>MGHHHHHHMPFAARLNTPMGPGRTVVVKGEVNANAKSFNVDLLAGKSKDIALHLNPRLNIKAFVRNSFLQESWGEEERNITSFPFSPGMYFEMIIYCDVREFKVAVNGVHSL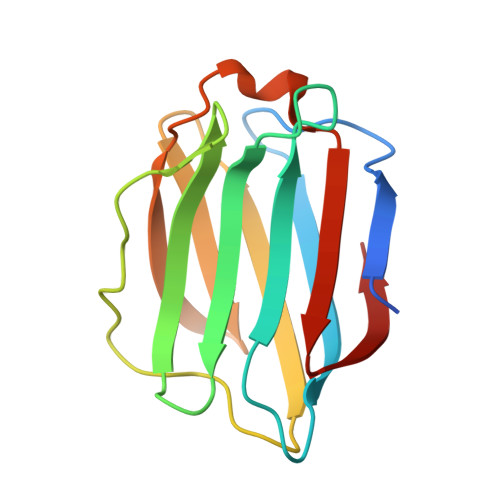EYKHRFKELSSIDTLEINGDIHLLEVR[4x]>[4x]GPNLDFQALEETTEYDGGYTRDSV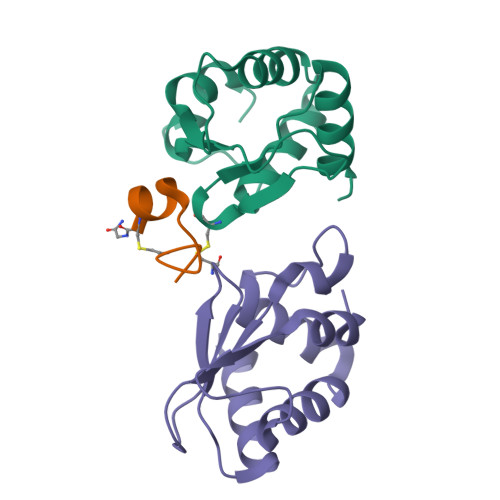LIREFWEIVHSFTDEQKRLFLQFTTGTDRAPVGGLGKLKMIIAKNGPDTERLPTSHTCFNVLLLPEYSSKEKLKERLLKAITYAKGFGML>WGSSTQALTYHQALTHSLQLCGVADHIKTFRPQCLVMTGAPNSRPAILHLVHAFTKNVGLMLCGHVRISSRRPNFKELNSDMLRYQRWLLNNNSKAFYTCVVAEDLRQGTQYMLQAAGLGRLRPNTLVIGFKNDWRIGDIKEVETYINLIHDAFDFQYGVVILRLREGLDISHIQGQDDSSGMKDVVVSVDISKDSDGDSSKPSSKATSVQNSPAVQKDKKSPTVP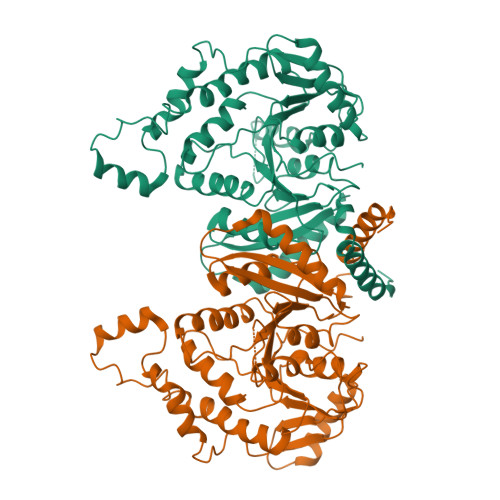LNVADQRLLDSQQFQQKQGKGTVDVWWLFDDGGLTLLIPYLIANKKKWKDCKIRVFIGGKINRIDHDRRAMATLLSKFRIDFSDITVLGDINTKPKSEGLTEFAEMIEPYKLREDDMEQEAAEKLKSEEPWRITANELELYKAKGNRQIRLNELLKEHSSTANLIVMSMPLARKGAVSSALYMAWLDTLSKDLPPILLVRGNHQSVLTFYS[2x]>MLDEALMPKHIALIMDGNRRWAKDKGLDVSEGYKHLFPKLKEICDISSKLGIQVITAFAFSTENWKRAKGEVDFLMQMFEELYDEFSRSGVRVSIIGCKTDLPMTLQKCIALTEETTKGNKGLHLVIA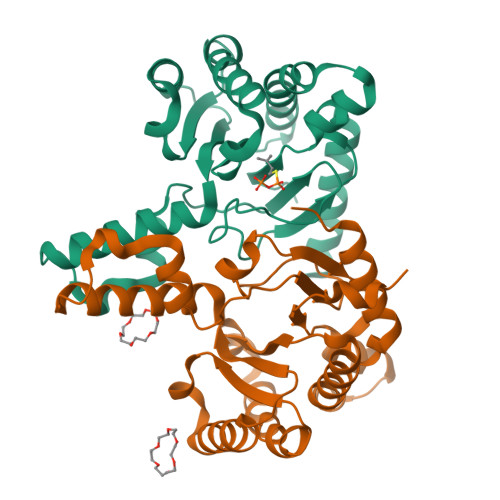LNYGGYYDILQATKSIVNKAMNGLLDVEDINKNLFDQELESKCPNPDLLIRTGGDQRVSNFLLWQLAYTEFYFTKTLFPDFGEEDLKEAIINFQQRHRRFGGHTY[2x]> QNRTVKGTVISSEDNEPLIGANVVVVGNTTIGAATDLDGNFTLSVPANAKMLRVSYSGMTTKEVAIANVMKIVLDPDSKVLEQVVVLGYGTGQKLSTVSGSVAKVSSEKLAEKPVANIMDALQGQVAGMQVMTTSGDPTAVASVEIHGTGSLGASSAPLYIVDGMQTSLDVVATMNPNDFESMSVLKDASATSIYGARAANGVVFIQTKKGKMSERGRITFNASYGISQILNTKPLDNMMTGDELLDFQVKAGFWGNNQTVQKVKDMILAGAEDLYGNYDSLKDEYGKTLFPVDFNHDADWLKALFKTAPTSQGDISFSGGSQGTSYYASIGYFDQEGMAREPANFKRYSGRLNFESRINEWLKVGANLSGAIANRRSADYFGKYYMGSGTFGVLTMPRYYNPFDVNGDLADVYYMYGATRPSMTEPYFAKMRPFSSESHQANVNGFAQITPIKGLTLKAQAGVDITNTRTSSKRMPNNPYDSTPLGERRERAYRDVSKSFTNTAEYKFSIDEKHDLTALMGHEYIEYEGDVIGASSKGFESDKLMLLSQGKTGNSLSLPEHRVAEYAYLSFF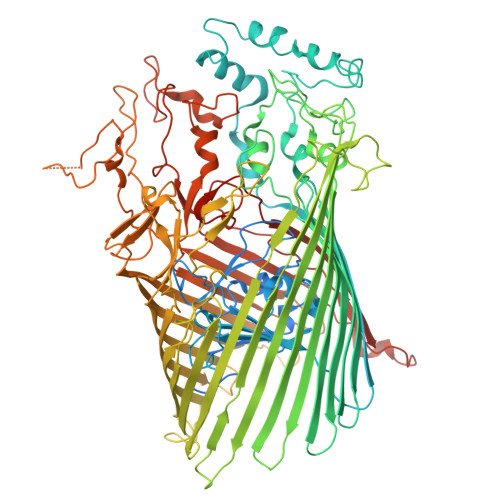SRFNYGFDKWMYIDFSVRNDQSSRFGSNNRSAWFYSVGGMFDIYNKFIQESNWLSDLRLKMSYGTTGNSEIGNYNHQALVTVNNYTEDAMGLSISTAGNPDLSWEKQSQFNFGLAAGAFNNRLSAEVDFYVRTTNDMLIDVPMPYISGFFSQYQNVGSMKNTGVDLSLKGTIYQNKDWNVYASANFNYNRQEITKLFFGLNKYMLPNTGTIWEIGYPNSFYMAEYAGIDKKTGKQLWYVPGQVDADGNKVTTSQYSADLETRIDKSVTPPITGGFSLGASWKGLSLDADFAYIVGKWMINNDRYFTENGGGLMQLNKDKMLLNAWTEDNKETDVPKLGQSPQFDTHLLENASFLRLKNLKLTYVLPNSLFAGQNVIGGARVYLMARNLLTVTKYKGFDPEAGGNVGKNQYPNSKQYVAGIQLSF> XADVAGTSNRDFRGREQRLFNSEQYNYNNSLNGEVSVWVYAYYSDGSVLVINKNSQYKVGISETFKALKEYREGQHNDSYDEYEVNQSIYYPNGGDARKFHSNAKPRAIQIIFSPSVNVRTIKMAKGNAVSVPDE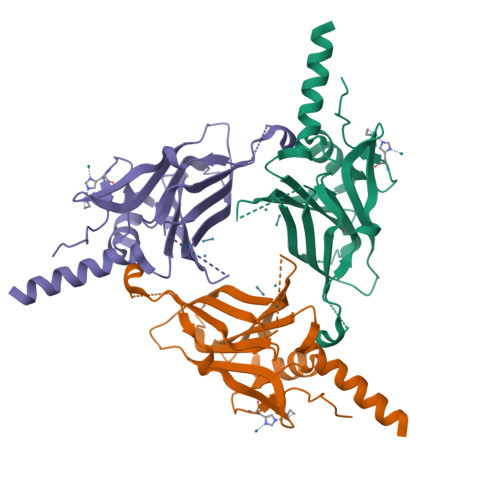YLQRSHPWEATGIKYRKIKRDGEIVGYSHYFELPHEYNSISLAVSGVHKNPSSYNVHNVMDVFQSCDLALRFCNRYWAELELVNHYISPNAYPYLDINNHSYGVALSNRQ> ADSVIKSDFSSL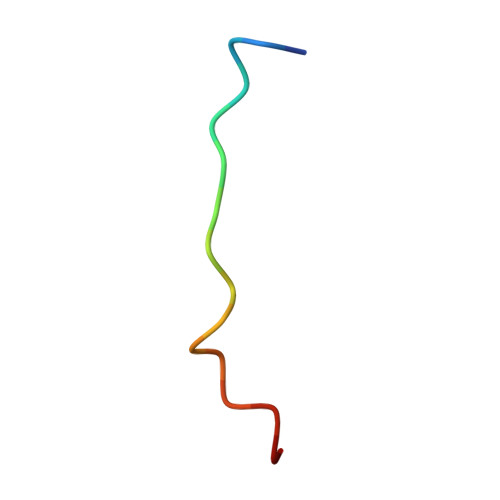KLDV> MDKFRVYGQSRLSGSVNISGAKNAALPILFAAILATEPVKLTNVPELKDIETTLKILRQLGVVVDRDATGAVLLDASNINHFTAPYELVKTMRASIWALAPLVARFHQGQVSLPGGCSIGARPVDLHISGLEKLGADIVLEEGYVKAQVSDRLVGTRIVIEKVSVGATLSIMMAATLAKGTTVIENAAREPEIVDTADFLNKMGAKITGAGSAHITIEGVERLTGCEHSVVPDRIETGTFLIAAAISGGCVVCQNTKADTLDAVIDKLREAGAQVDVTENSITLDMLGNRPKAVNIRTAPHPGFPTDMQAQFTLLNM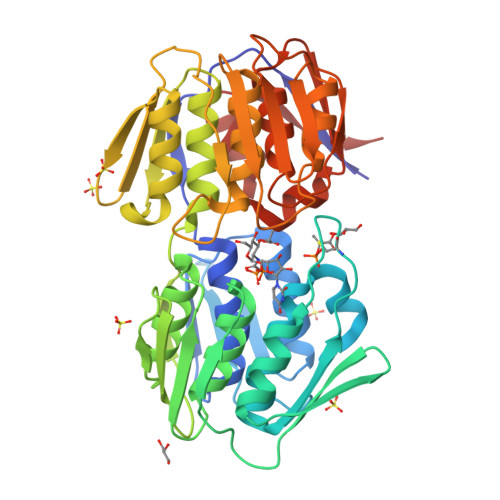VAEGTSIITETIFENRFMHIPELIRMGGKAEIEGNTAVCHGVEQLSGTEVIATDLRASISLVLAGCIATGETIVDRIYHIDRGYEHIEDKLRGLGAKIERFSGSDEA>[4x]LKNLNYSVPEEQGAGTVIGNIGRDARLQPGLPPAERGGGGRSKSGSYRVLENSAPHLLDVDADSGLLYTKQRIDRESLCRHNAKCQLSLEVFANDKEICMIKVEIQDINDNAPSFSSDQIEMDISENAAPGTRFPLTSAHDPDAGENGLRTYLLTRDD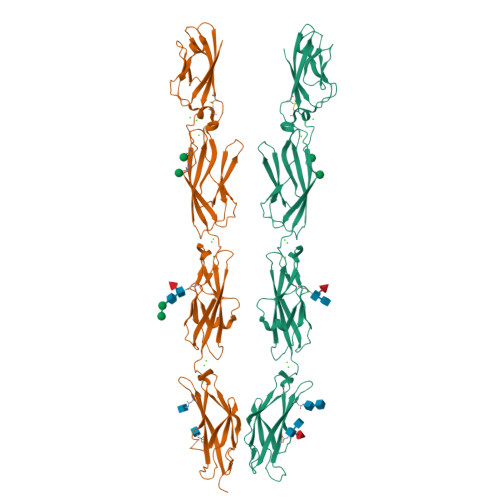HGLFGLDVKSRGDGTKFPELVIQKALDREQQNHHTLVLTALDGGEPPRSATVQINVKVIDSNDNSPVFEAPSYLVELPENAPLGTVVIDLNATDADEGPNGEVLYSFSSYVPDRVRELFSIDPKTGLIRVKGNLDYEENGMLEIDVQARDLGPNPIPAHCKVTVKLIDRNDNAPSIGFVSVRQGALSEAAPPGTVIALVRVTDRDSGKNGQLQCRVLGGGGTGGGGGLGGPGGSVPFKLEENYDNFYTVVTDRPLDRETQDEYNVTIVARDGGSPPLNSTKSFAIKILDHHHHHH>[2x]MAYQTIYPYTNEVLHTFDNM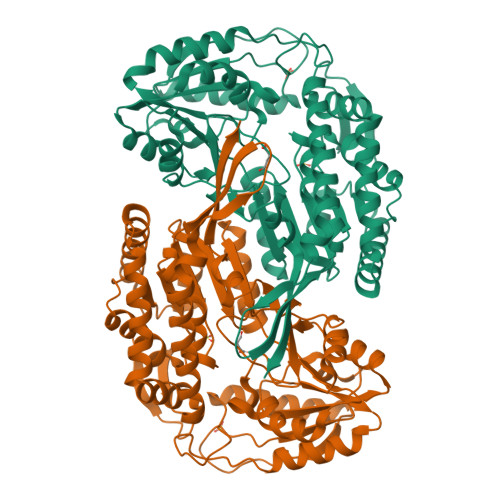TDQGLADVLERAHLLYKKWRKEDHLEERKAQLHQVANILRRDRDKYAEIMTKDMGKLFTEAQGEVDLCADIADYYADKADEFLMSTPLETDSGQAYYLKQSTGVILAVEPWNFPYYQIMRVFAPNFIVGNPMVLKHASICPRSAQSFEELVLEAGAEAGSITNLFISYDQVSQVIADKRVVGVCLTGSERGGASIAEEAGKNLKKTTLELGGDDAFIILDDADWDQLEKVLYFSRLYNAGQVCTSSKRFIVLDKDYDRFKELLTKVFKTAKWGDPMDPETTLAPLSSAQAKADVLDQIKLALDHGAELVYGGEAIDHPGHFVMPTIIAGLTKDNPIYYQEIFGPVGEIYKVSSEEEAIEVANDSNYGLGGTIFSSNQEHAKAVAAKIETGMSFINSGWTSLPELPFGGIKHSGYGRELSELGFTSFVNEHLIYIPNKTNNSNTKV>[3x]HDDHDHDHAHGSLGKHEHGVAQLNVALDGKTLELELDSPAMNLVGFEHAASTDADKAAVAKARAQLEKPLELFALPVTAG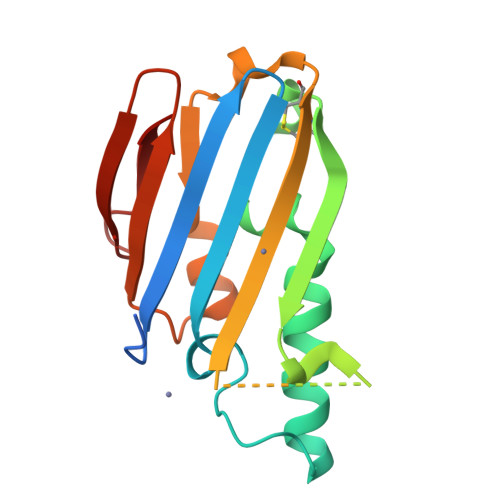CSVASQELRSPLFGDKAPAHAHKEKAGHEHEHEHEHEHGHADIHAHYQLSCEKPELLKLLTLAEFFKRFPATQKIQVQLIGPDGQKGADLAPASAELKL>MELIKGQALFLELDKKDFLSLKNNDKNIPTFAHPKNQEKILAIFSLPYKNP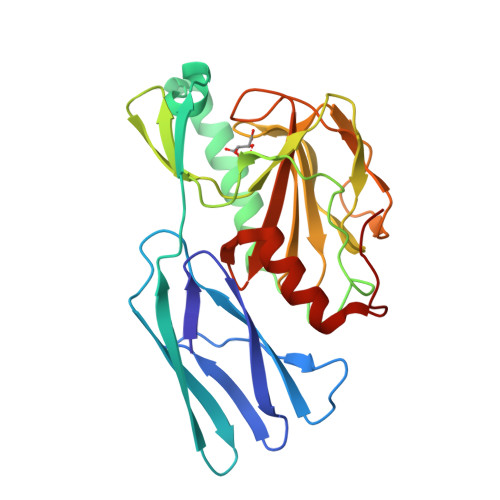PQNTKLIAFYKDKKEEIFIKTLEGNYKSEKLQVENKKIFPPKTIQERIAKELKEANAIYSSYTPKALFNGAFNIPLNSFITSDFGKARTFNEKVASYHSGTDFRAATGTPIYAANSGVVKIAKDRYFAGNSVVIDHGFGIYSQYYALSKIDVKVGQKIKKGELIGLSGASGRVSGPHLHFGILAGGKQVDPLDFVSKFNAIFQLEHHHHHH[3x]>[2x]MSSSTDNFSATMRDGLSNLARRLRFAMKEGSIWLGEQRMILLHTAALGALRKELVDTLGMERARGLFMRMGFHSGVRDAELAKTMRSGHSDFGMLEMGPCLHTIEGVVRVTPLTVDINIAAG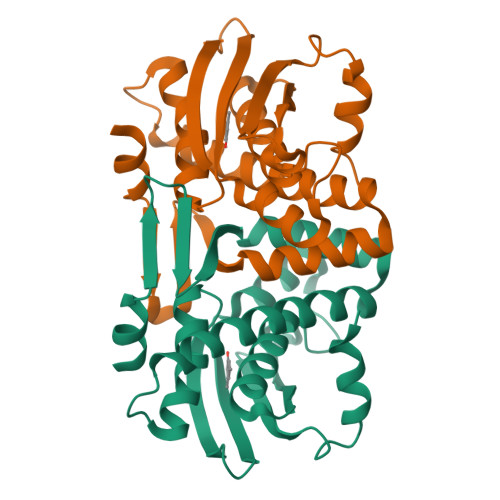VYHGEFLWEDSFEGDVHRQMFGVAQAPVCWMQIGYATGYTSALMGKTILYRELECVGCGHPHCRILGKPLEQWEDGEAELALYQPDPVI>[2x]MDYTPHTEEEIREMLRRVGAASLEDLFAHLPKEILSPPIDLPEPLPEWKVLEELRRLAAQNLPAHKAFLGGGVRSHHVPPVVQALAARGEFLTAYTPYQPEVSQGVLQATFEYQTMIAELAGLEIANASMYDGATALAEGVLLALRETGRMGVLVSQGVHPEYRAVLRAYLEAVGAKLLTLPLEGGRTPLPEVGEEVGAVVVQNPNFLGALEDLGPFAEAAHGAGALFVAVADPLSLGVLKPPGAYGADIAVGDGQSLGLPMGFGGPHFGFLATKKAFVRQLPGRLVSETVDVEG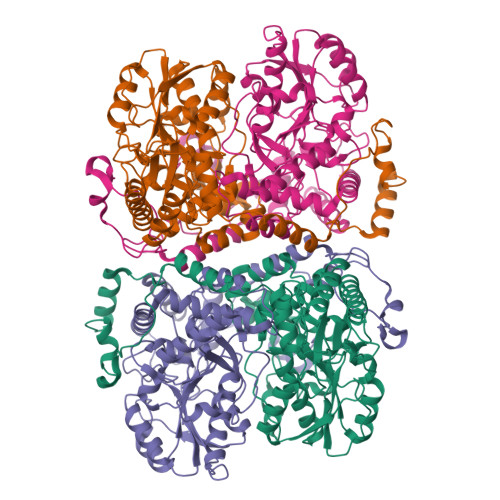RRGFILTLQAREQYIRRAKAKSNITTNAQLTALMGAMYLAALGPEGLREVALKSVEMAHKLHALLLEVPGVRPFTPKPFFNEFALALPKDPEAVRRALAERGFHGATPVPREYGENLALFAATELHEEEDLLALREALKEVLA;>[2x]MSFPLIFERSRKGRRGLKLVKAVPKAEDLIPKEHLREVPPRLPEVDELTLVRHYTGLSRRQVGVDTTFYPLGSCTMKYNPKLHEEAARLFADLHPYQDPRTAQGALRLMWELGEYLKALTGMDAITLEPAAGAHGELTGILIIRAYHEDRGEGRTRRVVLVPDSAHGSNPATASMAGYQVREIPSGPEGEVDLEALKRELGPHVAALMLTNPNTLGLFERRILEISRLCKEAGVQLYYDGANLNAIMGWARPGDMGFDVVHLNLHKTFTVPHGGGGPGSGPVGVKAHLAPYLPVPLVERGEEGFYLDFDRPKSIGRVRSFYGNFLALVRAWAYIRTLGLEGLKKAAALAVLNARYLKELLKEKGYRVPYDGPSMHEFVAQPPEGFRALDLAKGLLELGFHPPTVYFPLIVKEALMVEPTETEAKETLEAFAEAMGALLKKPKEWLENAPYSTPVRRLDELRANKHPKLTYFDEG>XXXXXXXXXXXXEEQRRKKRRLKKRIFAAVSEGCVEELVELLVELQELCRRRHDEDVPDFLMHKLTASDTGATCLMKALLNINPNTKEIVRILLAFAEENDILGRFINAEYTEEAYEGQTALNIAIERRQGDIAALLIAAGADVNAHAKGAFFNPKYQHEGFYFGETPLALAACTNQPEIVQLLMEHEQTDITSRDSRGNNILHALVTVAEDFKTQNDFVKRMYDMILLRSGNWELETTRNNDGLTPLQLAAKMGKAEILKYILSREIKEKRLRSLSRKFTDWAYGPVSSSLYDLTNVDTTTDNSVLEITVYNTNIDNRHEMLTLEPLHTLLHMKWKKFAKHMFFLSFCFYFFYNITLTLVSYYRPREEEAIPHPLALTHKMGWLQLLGRMFVLIWAMCISVKEGIAIFLLRPSDLQSILSDAWFHFVFFIQAVLVILSVFLYLFAYKEYLACLVLAMALGWANMLYYTRGFQSMGMYSVMIQKVILHDVLKFLFVYIVFLLGFGVALASLIEKCPKDNKDCSSYGSFSDAVLELFKLTIGLGDLNIQQNSKYPILFLFLLITYVILTFVLLLNMLIALMGETVENVSKESERIWRLQRARTILEFEKMLPEWLRSRFRMGELCKVAEDDFRLCLRINEVKWTEWKTHVSFLNEDPGPVRRTDFNKIQDSSRNNSKTTLNAFEEVEEFPETSVVDAGLEVLFQGDYKDDDDKAHHHHHH[4x]

The Transient Receptor Potential Vanilloid (TRPV) channel subfamily is a subset of the large TRP channel superfamily, and consist of subtypes TRPV1-TRPV6. TRPV1-4 are intrinsically temperature sensitive (thermoTRPV) and have been found to play important roles in numerous physiological processes including thermosensation, nociception, and osmosensation. TRPV3 exhibits use-dependent increase in current amplitudes (termed sensitization) upon repeated applications of either ligand or heat. The combination of our structural data and functional experiments provides evidence that hysteresis, sensitization, and activation of TRPV3 involves increased coupling between structural elements from the cytoplasmic (ARD and CD) and the transmembrane domains (TRP and S6) is triggered by a coil-to-helix transition in the distal CTD.

Inspection of this structure revealed that TRPV3 undergoes conformational changes in both the transmembrane (TM) and cytoplasmic domains in the presence of ligand. The cryo-EM map of TRPV3K169A 2-APB contains non-protein densities between the TRP domain and the Pre-S1CD in all four protomers. Because a previous high-throughput mutagenesis study identified this site as critical for 2-APB binding, we assigned the non-protein densities as 2-APB. The 2-APB molecule is nestled amongst residues W692, R693 and R696 in the TRP domain and H417, H426, H430 and W433 in the Pre-S1CD. Notably, a comparison of S6 helices from the closed TRPV3WT and TRPV3K169A 2-APB shows that the linker region between the S6 helix and the TRP domain also changes: while the two helices are connected via a loose loop in the TRPV3WT structure, they form a single helical structure in TRPV3K169A 2-APB, suggestive of increased coupling between the TRP domain and S6 upon 2-APB binding. In addition, the TRP domain of TRPV3K169A 2-APB undergoes a swivel relative to the S6 helix. Namely, the swivel in the TRP domain can be traced back to changes in coupling between the loop of AR5, the HLHCD and the TRP domain which are induced by the coil-to-helix transition in the distal CTD. However, in TRPV3K169A 2-APB, where the coil-to-helix transition in the distal CTD has enforced a conformational change in the loop of AR5, AR5 interacts with the HLHCD. Notably, 2-APB binding between the Pre-S1CD and the TRP domain appears to further increase the coupling between the CD and the TRP domain, suggesting a mechanism for 2-APB-dependent activation of TRPV3.>M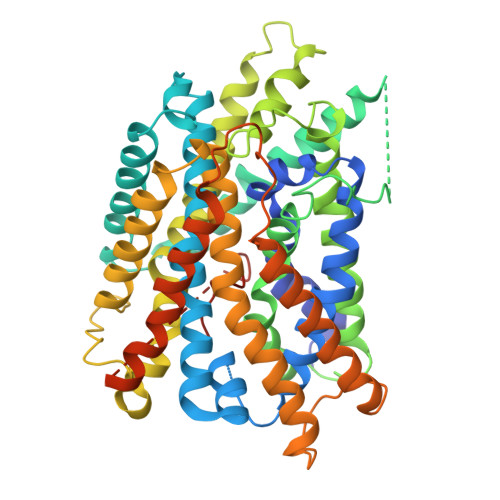ATSVQTGKAKQLTLLGFFAITASMVMAVYEYPTFATSGFSLVFFLLLGGILWFIPVGLCAAEMATVDGWEEGGVFAWVSNTLGPRWGFAAISFGYLQIAIGFIPMLYFVLGALSYILKWPALNEDPITKTIAALIILWALALTQFGGTKYTARIAKVGFFAGILLPAFILIALAAIYLHSGAPVAIEMDSKTFFPDFSKVGTLVVFVAFILSYMGVEASATHVNEMSNPGRDYPLAMLLLMVAAICLSSVGGLSIAMVIPGNEINLSAGVMQTFTVLMSHVAPEIEWTVRVISALLLLGVLAEIASWIVGPSRGMYVTAQKNLLPAAFAKMNKNGVPVTLVISQLVITSIALIILTNTGGGNNMSFLIALALTVVIYLCAYFMLFIGYIVLVLKHPDLKRTFNIPGGKGVKLVVAIVGLLTSIMAFIVSFLPPDNIQGDSTDMYVELLVVSFLVVLALPFILYAVHDRKGKANTGVTLEPINSQNAPKGHFFLHPRARSPHYIVMNDKKH[2x]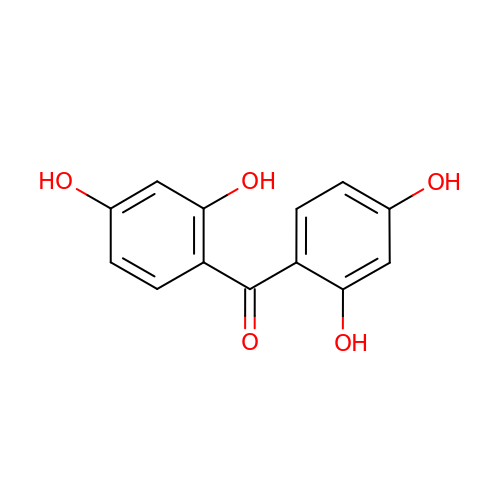bis(2,4-dihydroxyphenyl)methanone | C13 H10 O5 | WXNRYSGJLQFHBR-UHFFFAOYSA-N> MLFEMTPETFKKVNSSNRIIKGLQYTPLASSIPLENGLQNVLYPSSKFQNEPLQLNSEESSIMQRYVDMLNPGATFVNDSETFNFYKNALSAMITEPAMPAMRVNASPVLDQKVCNSDSLSELNDFTKSLIQPSMLMCEPKEKPDASSINTNRSSSDNGFLTPSSSPRSPSCSRVFNAVQLCSPKKSKDDITTPKKRLMEDTYSPRESPSKIQRLQDVLLKQLQDTRLLISQVIEAENSEDFSSNSLFIKREDDDGKHISSHAIEKLYMALTKLSRLGACDKLLEEGSIILVKQILEKELKELPVACYSIINLHDSLTQFPNLDFILKTTALVLFIIFLVPSFKKLQNEESILHLLNILHSIFEYTVPEAIDNIVQSKTSDARTSEIQHLSVLLQKVANVLNILSKVAHEIPLSEAVVIRIVYLFPKVSTLDNSFKTKLPNCNSSSFDFLKAPLFQTLQYLFRLYPYQRDFIIEESLTNFSHLPTARSVSRTYRLSNGKSIQYYSTLFVRLIQSCSIQNLFDSEIVQSESKSTEALHSGNLTEHLKTVESILSKSRHEEYRIANHIVAYLLSRSLKQNKTESDNSFAILTKILLEDLLNMLSLPEWCGTETIIRQFAMNLVMTVTNDKQAVSSKNAALDLISLIVNKVLALFDLSLFEKHNIPAPTNFNDIISFIPSITRLNELSQVSFNHFYFLCKGDISLENILPYNYNKWFSFLLQLRKVCNDSEALKIIDNCIDKNMQKSQEGFQGPSPFKADENDEDIFIISLYHSSLFLNLKFFVSLIIGFLDSPQASLRTKCLRIINQMKTIPSILRTHPEVLAQIISKSNDQSAIVRDTVLDLLGTYIMAYRETIPQIYGCIISGISDPSTIVRKRAIKQLCEVYEATEDLNIRVDIASKLLTRSNDEEETISELSLEVLEKLWFSPASNELDCQKGYEQLTFLEKQKLRVQYFPILKLCAEPSTERHVLLVTSLKTMLTSKEEINLSTLHTQIRLLLSCLFNQLIEVVT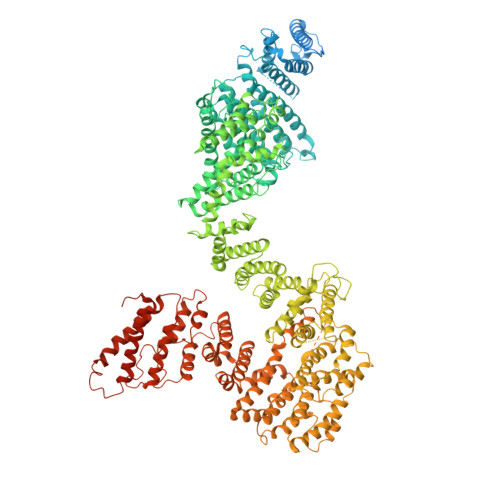EDQVDESTKGILYEIMSTLFVFSRAFPFLFDLSYLHLLKPYLRSASTIEEQRFLYYVVAIFRQVLPFQKEISESFLRSLESVLLQRLTKAGTATLMEIVPCLCSLFTRLNDYERLKKIVVSCLKSLEEARHSENNFQKMVRLIDLIGLFSRYGDLNRINDDWKHSLDFISPECDDAYVILLGYFQKLLKDAKGQLRIHIIDNMSRICLRETSLFISPLMLSTLDMIIAENNVNEVSVLFKSFLELLAADEDLIFEADQKLSLKGKQNVQSNKSVDRDMLKGTKDKQWIEGVSASLMQHFLPCILDSCFSKNLRYSMLGIEILKCIIHQGLVNPRMCFSTIIALESNAIKETREVAILLHTELHRRHESLIDGLYAQSADLIFSLQKTEEYQTFKLGEFSPFQSAYTIVSADKSSKSRKKLIMQILKPLKLDGIDLPSFTEEKVSFVSFCCVCLAGIPYVSIEEPLMIISTVDSVLATIGPTITGWMKKLDHERFKILAGINLCNLIYLKRYIKYAFSISDSSRPIREKKPLTLLNRGYVDLITSDAKPDIVSKLVIKLFEEENILSGEDQVEGEQLTVV> MTDQAFVTLTTNDAYAKGALVLGSSLK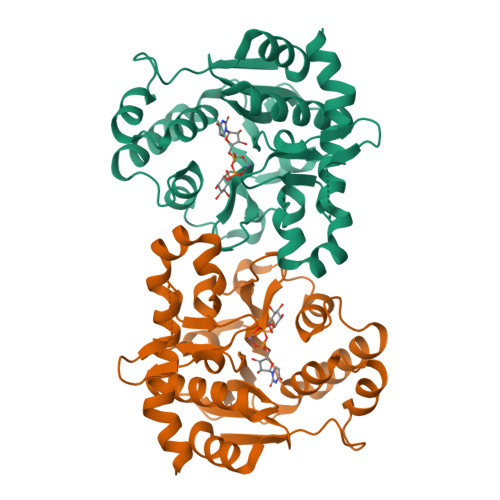QHRTSRRLAVLTTPQVSDTMRKALEIVFDEVITVDILDSGDSAHLTLMKRPELGVTLTKLHCWSLTQYSKCVFMDADTLVLANIDDLFEREELSAAPDPGWPDCFNSGVFVYQPSVETYNQLLHVASEQGSFDGGDQGLLNTFFNSWATTDIRKHLPFIYNLSSISIYSYLPAFKAFGANAKVVHFLGQTKPWNYTYDTKTKSVRSEGHDPTMTHPQFLNVWWDIFTTSVVPLLQQFGLVQDTCSYQHVEDVSGAVSHLSLGETPATTQPFVSSEERKERWEQGQADYMGADSFDNIKKKLDTYLQ D2-BGL is a GH3 β-glucosidase from the indigenous Taiwanese fungus Chaetomella raphigera. Endo-glucanases (EC 3.2.1.4) break down internal 1,4 β-glycosidic bonds in the cellulose chain, and exo-glucanases (including β-1,4-glucan cellobiohydrolase EC 3.2.1.91 and 1,4-β-d-glucan glucohydrolase EC 3.2.1.74) digest the chain endings to release cellobiose. β-Glucosidases (EC 3.2.1.21) finalize the cellulolytic process by hydrolyzing cellobiose into glucose. Crystal structure analysis revealed that D2-BGL belongs to glycoside hydrolase (GH) family 3. D2-BGL has the classical three-domain structure of a GH3 β-glucosidase: a TIM barrel-like domain (residues 1–307), an α/β sandwich domain (residues 319–521), and a fibronectin type III-like domain (residues 573–712).

There are three intra-domain disulfide bonds involving residues C39–C55, C199–C210 and C369–C374. Three N-glycosylation sites (N68, N205 and N273) were determined by the presence of N-acetylglucosamine after endoglycosidase H (Endo H) treatment, and one O-linked mannose was observed on residue T431. The N68 and T431 glycosylation sites have not been observed in crystal structures of other reported GH3 β-glucosidases. In D2-BGL, residues D232 and E442 are nucleophile and general acid/base residues, respectively. D58, R122, K155, H156 and W233 form the substrate-binding subsite −1. The hydrophobic substrate-binding subsite +1 is formed by W34, Y444 and F256. Structure alignment revealed that all key amino acid residues lie in the same positions for both D2-BGL and AaBGL1, except for the phenylalanine involved in substrate-binding subsite +1 (i.e., F256 in D2-BGL and F305 in AaBGL1), in which the two aromatic rings have different orientations. The connection loop between the TIM barrel-like domain and the α/β sandwich is shorter in D2-BGL than in AaBGL1 (12 a.a. from residues 307 to 318 vs 29 a.a. from residues 356 to 384). This loop plays a role in forming protein dimer in AaBGL1, but we did not observe that dimerization state for the D2-BGL crystal structure. Another short loop is close to the active site entry region in D2-BGL (3 a.a. from residues 166 to 168), which may influence the efficiency of enzyme catalysis by broadening the active site pocket.

> PGDGDWAAAYKKATAALAKLSNTDKASIVTGVGWEKGPCVGNTAAVASIGLPELCYQDGPLGIRFVQNVTAFPTGIQTASTWDISLIYSRGLALGQEAKALGINVQLGPVAGPIGKIPEAGRNWEGFSPDPYLNGLAMSNTITGMQDAGVQACAKHFIGNEQETNRDTMSSNIDDRTFHELYLWPFADAIKANVASIMCSYNKFNETYACENNFLTTILKGELDFQGFVVSDWAAQHTTIGSANAGLDVAMPGDNFGDNYYLWGSNLLAAISNGTVAQSRLDDMVTRILASWYFVGQDQGYPAVTWSSWNGGLGGPNVQADHKQVARAIARDGIVLLTNKNKALPLKKPASLAIIGQDAIDNPAGINSCSDRGCDTGHLAMGWGSGTADFPYLVAPLDAITPLAQAQGTKLVLSTTDSTSAAASAAAAAETAIVFITADSGEGYITVDGQLGDRNSLAPWNNGTALVQAVASASKNVIVVINSVGPLILEDILALSSVKAIVWAGVSGQESGNGLADILYGSVSPSGKLPYTIAKQASDYGTAIVPGDDNFPEGLFVDYRHFDQANIQPRFEFGYGLSYTTFQYSQLTAKYSDTSAGSSTLAPGGPKGLYDIVATVTAKVTNSGTVSGAEVAQLYIGLPGSAPASPPKQLRGFDKISLKPGKSGTVTFNLRRKDLSYWDTASAQWVTPTSGEFSLYVGASSRDIRLQGSLKCSGQGIRKGGH>GAMNAQAEEFKKYLETNGIKPKQFHKKELIFNQWDPQEYCIFLYDGITKLTSISENGTIMNLQYYKGAFVIMSGFIDTETSVGYYNLEVISEQATAYVIKINELKELLSKNLTHFFYVFQTLQKQVSYSLAKFNDFSINGKLGSICGQLLILTYVYGKETPDGIKITLDNLTMQELGYSSGIAHSSAVSRIISKLKQEKVIVYKNSCFYVQNLDYLKRYAPKLDEWFYLACPATWGKLN[2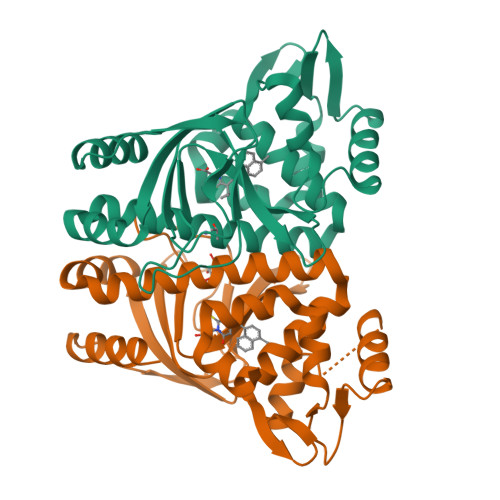x]>[4x]MDSLDQCIVNACKNSWDKSY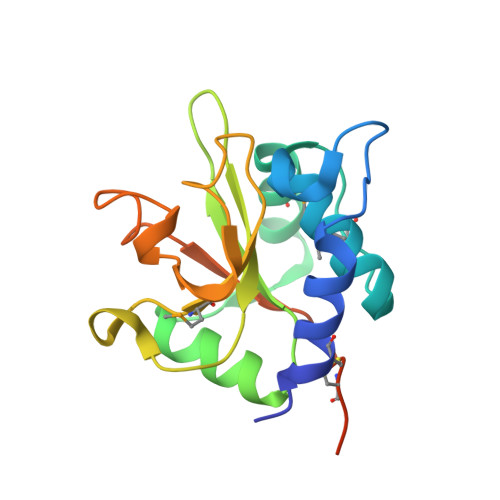LAGTPNKDNCSGFVQSVAAELGVPMPRGNANAMVDGLEQSWTKLASGAEAAQKAAQGFLVIAGLKGRTYGHVAVVISGPLYRQKYPMCWCGSIAGAVGQSQGLKSVGQVWNRTDRDRLNYYVYSLASCSLPRASAAALEHHHHHH(2R)-2-hydroxy-7-methoxy-2-(pentafluoroethyl)-2,3-dihydro-4H-1-benzopyran-4-one | C12 H9 F5 O4 | 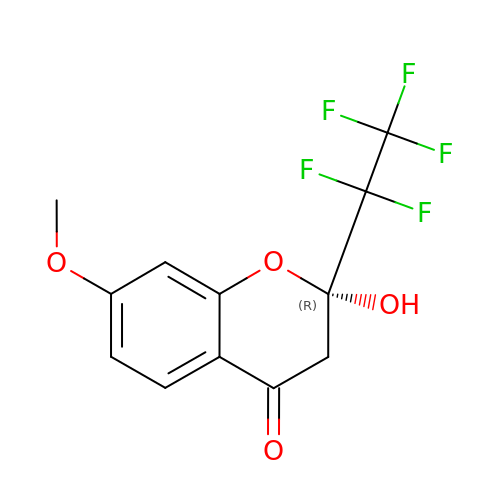NQJASZMLBMBHRG-SNVBAGLBSA-N> MSLLERGLSKLTLNAWKDREGKIPAGSMSAMYNPETIQLDYQTRFDTEDTINTASQSNRYVISEPVGLNLTLLFDSQMPGNTTPIETQLAMLKSLCAVDAATGSPYFLRITWGKMRWENKGWFAG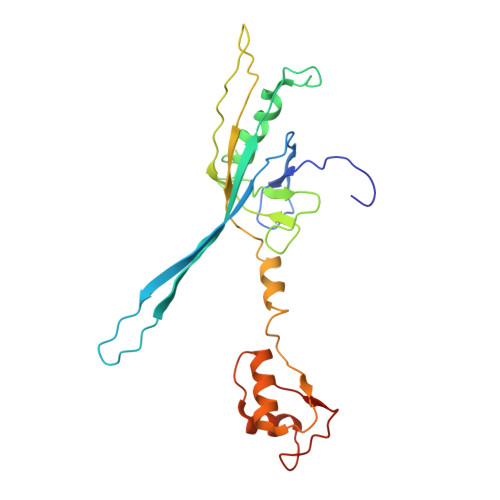RARDLSVTYTLFDRDATPLRATVQLSLVADESFVIQQSLKTQSAPDRALVSVPDLASLPLLALSAGGVLASSVDYLSLAWDNDLDNLDDFQTGDFLRATKGEEV>MRVLALSAVFLVASIIGMPAVAKEWQENKSWNAHFTEHKSQGVVVLWNENKQQGFTNNLKRANQAFLPASTFAIPNSLIALDLGVVKDEHQVFKWDGQTRDIATWNRDHNLITAMKYSVVPVYQEFARQIGEARMSKMLHAFDYGNEDISGNVDSFWLDGGIRISATEQISFLRKLYHNKLHVSERSQRIVKQAML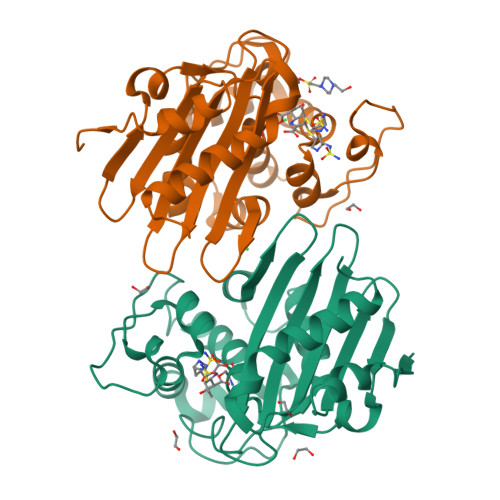TEANGDYIIRAKTGYSTRIEPKIGWWVGWVELDDNVWFFAMNMDMPTSDGLGLRQAITKEVLKQEKIIP[2x]PTPN21 belongs to the four-point-one, ezrin, radixin, moesin (FERM) domain–containing protein tyrosine phosphatases (PTP) and plays important roles in cytoskeleton-associated cellular processes like cell adhesion, motility, and cargo transport. Because of the presence of a WPE loop instead of a WPD loop in the phosphatase domain, it is often considered to lack phosphatase activity. However, many of PTPN21’s biological functions require its catalytic activity. Combined with biochemical analysis, we have found that PTPN21 PTP is weakly active and is autoinhibited by association with its FERM domain.

To help crystallize the FERM-PTP complex, we generated a mini PTPN21, replacing the disordered region between the two domains with a flexible linker. After adjusting the linker length, we managed to crystalize the FERM-PTPC1108S complex and determined its structure at 3.0 Å. The mini PTPN21 structure showed that the FERM F1 lobe binds to the α3 and β5 regions of PTP and buries an area around 886 Å2. The interaction interface can be further divided into three parts. In the top part, highly conserved residues from FERM α1 region (R59, E57, R55, and Q54) interact with residues from PTP α3 (R1089, S1086, and E1083) through hydrogen bonds and electrostatic interactions. In the middle, FERM β2 forms an antiparallel β sheet with β5 from PTP, which is stabilized by main-chain hydrogen bonding and side-chain hydrophobic interactions. In the lower part, R1031 from PTP β5 is sandwiched between E42 and E47 from the FERM domain, and E42 also forms a hydrogen bond with N1019. Mutation of critical interface residues in either PTP (R1031A and R1089A) or FERM (E47A and E57A) abolished FERM-PTP association. Several mutations found in patients with cancer [E42K, R59Q, and R1089H, from The Cancer Genome Atlas (TCGA) and Catalogue Of Somatic Mutations In Cancer (COSMIC) databases] are located in the FERM-PTP interface. Normally, PTPN21 is in an auto-inhibited state, where the FERM domain interacts with the PTP domain and stabilizes the WPE loop in the open (inactive) conformation.

> ATNDERCKILEQRLEQGMVFTEYERILKKRLVDGECSTARLPENAERNRFQDVLPYDDVRVELVPTKENNTGYINASHIKVSVSGIEWDYIATQGPLQNTCQDFWQMVWEQGIAIIAMVTAEEEGGREKSFRYWPRLGSRHNTVTYGRFKITTRFRTDSGCYATTGLKMKHLLTGQERTVWHLQYTDWPEHGCPEDLKGFLSYLEEIQSVRRHTNSTSDPQSPNPPLLVHSSAGVGRTGVVILSEIMIACLEHNEVLDIPRVLDMLRQQRMMLVQTLCQYTFVYRVLIQFLKSSRLI;> SSKSCLVARIQLLNNEFVEFTLSVESTGQESLEAVAQRLELREVTYFSLWYYNKQNQRRWVDLEKPLKKQLDKYALEPTVYFGVVFYVPSVSQLQQEITRYQYYLQLKKDILEGSIPCTLEQAIQLAGLAVQADFGDFDQYESQDFLQKFALFPVGWLQDEKVLEEATQKVALLHQKYRGLTAPDAEMLYMQEVERMDGYGEESYPAKDSQGSDISIGACLEGIFVKHKNGRHPVVFRWHDIANMSHNKSFFALELANKEETIQFQTEDMETAKYIWRLCVARHKFYRLNQ>[2x]TPEMPVLENRAAQGDITAPGGARRLTGDQTAALRDSLSDKPAKNIILLIGDGMGDSEITAARNYAEGAGGFFKGIDALPLTGQYTHYALNKKTGKPDYVTDSAASATAWSTGVKTYNGALGVDIHEKDHPTILEMAKAAGLATGNVSTAELQDATPAALVAHVTSSKCYGPSATSEKCPGNALEKGGKGSITEQLLNARADVTLGGGAKTFAETATAGEWQGKTLREQAQARGYQLVSDAASLNSVTEAN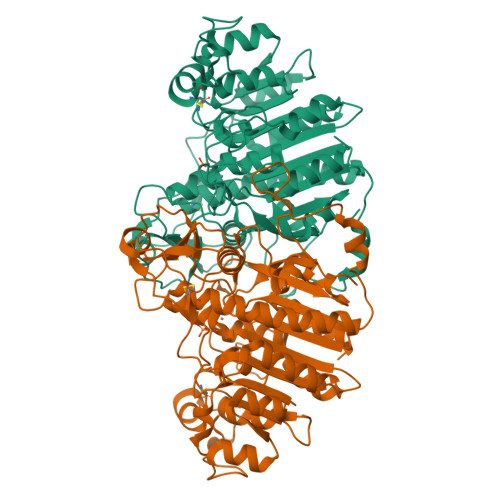QQKPLLGLFADGNMPVRWLGPKATYHGNIDKPAVTCTPNPQRNDSVPTLAQMTDKAIELLSKNEKGFFLQVEGASIDKQDHAANPCGQIGETVDLDEAVQRALEFAKKEGNTLVIVTADHAHASQIVAPDTKAPGLTQALNTKDGAVMVMSYGNSEEDSQEHTGSQLRIAAYGPHAANVVGLTDQTDLFYTMKAALGLK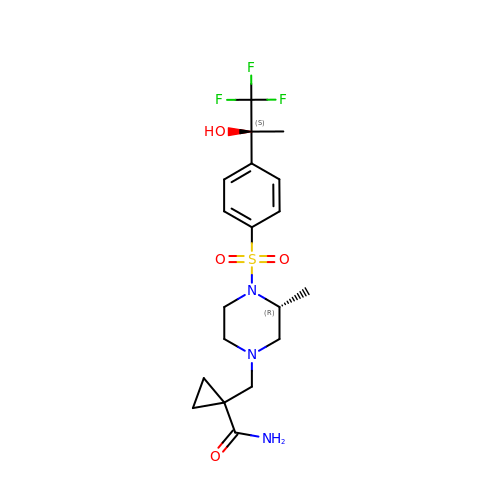1-{[(3R)-3-methyl-4-({4-[(1S)-2,2,2-trifluoro-1-hydroxy-1-methylethyl]phenyl}sulfonyl)piperazin-1-yl]methyl}cyclopropanecarboxamide | C19 H26 F3 N3 O4 S | YJFULAYRAKPBCY-DYVFJYSZSA-N>[4x]GPLGSRRRVRAILPYTKVPDTDEISFLKGDMFIVHNELEDGWMWVTNLRTDEQGLIVEDLVEEVGR;>[4x]MHHHHHHSSGRENLYFQGSVFGVPLTVNVQRTGQPLPQSIQQAMRYLRNHCLDQVGLFRKSGVKSRIQALRQMNEGAIDCVNYEGQSAYDVADMLKQYFRDLPEPLMTNKLSETF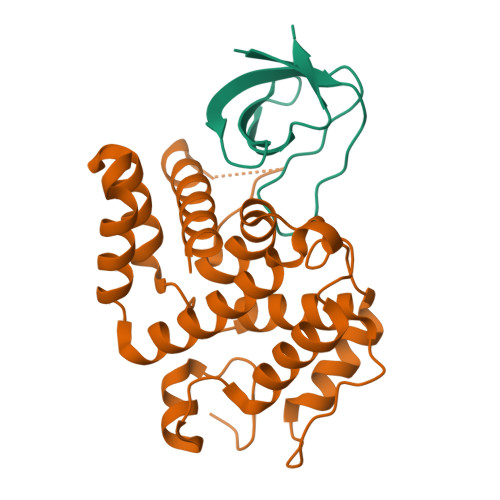LQIYQYVPKDQRLQAIKAAIMLLPDENREVLQTLLYFLSDVTAAVKENQMTPTNLAVCLAPSLFHLNTLKRENSSPRVMQRKQSLGKPDQKDLNENLAATQGLAHMIAECKKL> MSNNNTSIHDFDFSFICNYFKLLKRQGPGSPEATRKAVSFINELTDDAKIADIGCGTGGQTLFLADYVKGQITGIDLFPDFIEIFNENAVKANCADRVKGITGSMDNLPFQNEELDLIWSEGAIYN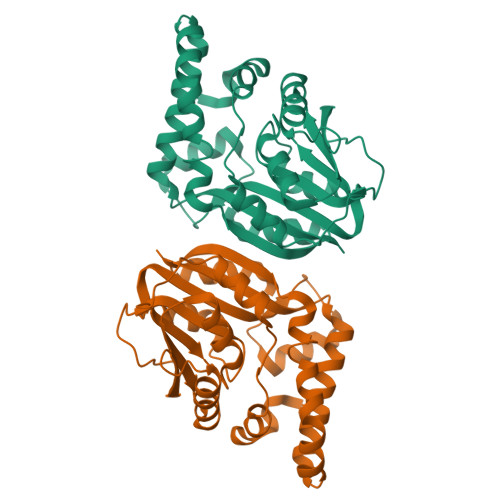IGFERGMNEWSKYLKKGGFIAVSEASWFTSERPAEIEDFWMDAYPEISVIPTCIDKMERAGYTPTAHFILPENCWTEHYFAPQDEVRETFMKEHAGNKTAMDFMKGQQYERSLYSKYKDYYGYVFYIGQKR>[60x]MPWWYRRRSYNPWRRRNWFRRPRKTIYRRYRRRRRWVRRKPFYKRKIKRLNIVEWQPKSIRKCRIKGMLCLFQTTEDRLSYNFDMYEESIIPEKLPGGGGFSIKNISLYA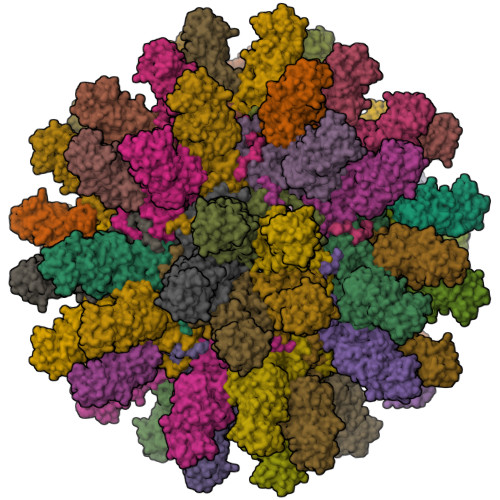LYQEHIHAHNIFTHTNTDRPLARYTGCSLKFYQSKDIDYVVTYSTSLPLRSSMGMYNSMQPSIHLMQQNKLIVPSKQTQKRRKPYIKKHISPPTQMKSQWYFQHNIANIPLLMIRTTALTLDNYYIGSRQLSTNVTIHTLNTTYIQNRDWGDRNKTYYCQTLGTQRYFLYGTHSTAQNINDIKLQELIPLTNTQDYVQGFDWTEKDKHNITTYKEFLTKGAGNPFHAEWITAQNPVIHTANSPTQIEQIYTASTTTFQNKKLTDLPTPGYIFITPTVSLRYNPYKDLAERNKCYFVRSKINAHGWDPEQHQELINSDLPQWLLLFGYPDYIKRTQNFALVDTNYILVDHCPYTNPEKTPFIPLSTSFIEGRSPYSPSDTHEPDEEDQNRWYPCYQYQQESINSICLSGPGTPKIPKGITAEAKVKYSFNFKWGGDLPPMSTITNPTDQPTYVVPNNFNETTSLQNPTTRPEHFLYSFDERRGQLTEKATKRLLKDWETK> TIDNPGLGNCAFYAFAIGLVNIIQEEAKYNRRTMFDRWVGLDRSISGQYDEILKLNLEDPDKELLDRLQSSLRIVTYQYQIRELRNVCVFRNGNYNRLTGNSNFVNFAALYYGDPLDTDSRFNPFADSVPILIKMANIDRDSVHPGHENDVLVPLFLDLLYGDTTNPADITLETEPKSDSPIITAMNNITQDFFWGTHLDLNYLAEAFEVNLHVLRNNSPIQEFVDIP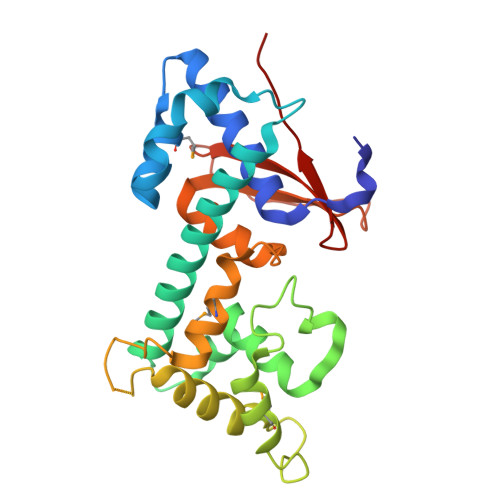ERHTLTLTNSNNTHWTTQITTAR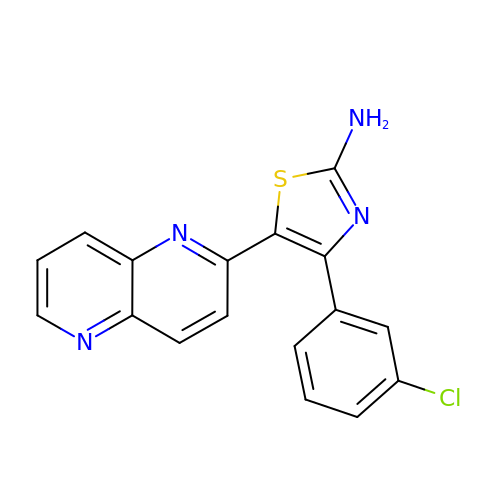4-(3-chlorophenyl)-5-(1,5-naphthyridin-2-yl)-1,3-thiazol-2-amine | C17 H11 Cl N4 S | JVXFJMXCRSAZFH-UHFFFAOYSA-N> MACWPQLRLLLWKNLTFRRRQTCQLLLEVAWPLFIFLILISVRLSYPPYEQHECHFPNKAMPSAGTLPWVQGIICNANNPCFRYPTPGEAPGVVGNFNKSIVARLFSDARRLLLYSQKDTSMKDMRKVLRTLQQIKKSSSNLKLQDFLVDNETFSGFLYHNLSLPKSTVDKMLRADVILHKVFLQGYQLHLTSLCNGSKSEEMIQLGDQEVSELCGLPREKLAAAERVLRSNMDILKPILRTLNSTSPFPSKELAEATKTLLHSLGTLAQELFSMRSWSDMRQEVMFLTNVNS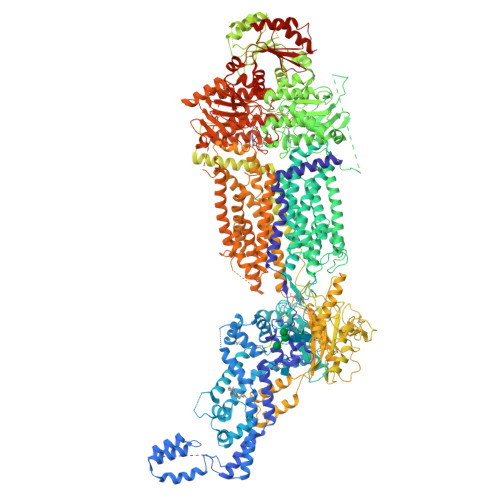SSSSTQIYQAVSRIVCGHPEGGGLKIKSLNWYEDNNYKALFGGNGTEEDAETFYDNSTTPYCNDLMKNLESSPLSRIIWKALKPLLVGKILYTPDTPATRQVMAEVNKTFQELAVFHDLEGMWEELSPKIWTFMENSQEMDLVRMLLDSRDNDHFWEQQLDGLDWTAQDIVAFLAKHPEDVQSSNGSVYTWREAFNETNQAIRTISRFMECVNLNKLEPIATEVWLINKSMELLDERKFWAGIVFTGITPGSIELPHHVKYKIRMDIDNVERTNKIKDGYWDPGPRADPFEDMRYVWGGFAYLQDVVEQAIIRVLTGTEKKTGVYMQQMPYPCYVDDIFLRVMSRSMPLFMTLAWIYSVAVIIKGIVYEKEARLKETMRIMGLDNSILWFSWFISSLIPLLVSAGLLVVILKLGNLLPYSDPSVVFVFLSVFAVVTILQCFLISTLFSRANLAAACGGIIYFTLYLPYVLCVAWRDYVGFTLKIFASLLSPVAFGFGCEYFALFEEQGIGVQWDNLFESPVEEDGFNLTTSVSMMLFDTFLYGVMTWYIEAVFPGQYGIPRPWYFPCTKSYWFGEESDEKSHPGSNQKRISEICMEEEPTHLKLGVSIQNLVKVYRDGMKVAVDGLALNFYEGQITSFLGHNGAGKTTTMSILTGLFPPTSGTAYILGKDIRSEMSTIRQNLGVCPQHNVLFDMLTVEEHIWFYARLKGLSEKHVKAEMEQMALDVGLPSSKLKSKTSQLSGGMQRKLSVALAFVGGSKVVILDQPTAGVDPYSRRGIWELLLKYRQGRTIILSTHHMDEADVLGDRIAIISHGKLCCVGSSLFLKNQLGTGYYLTLVKKDVESSLSSCRNSSSTVSYLKKEDSVSQSSSDAGLGSDHESDTLTIDVSAISNLIRKHVSEARLVEDIGHELTYVLPYEAAKEGAFVELFHEIDDRLSDLGISSYGISETTLEEIFLKVAEESGVDAETSDGTLPARRNRRAFGDKQSCLRPFTEDDAADPNDSDIDPESRETDLLSGMDGKGSYQVKGWKLTQQQFVALLWKRLLIARRSRKGFFAQIVLPAVFVCIALVFSLIVPPFGKYPSLELQPWMYNEQYTFVSNDAPEDTGTLELLNALTKDPGFGTRCMEGNPIPDTPCQAGEEEWTTAPVPQTIMDLFQNGNWTMQNPSPACQCSSDKIKKMLPVCPPGAGGLPPPQRKQNTADILQDLTGRNISDYLVKTYVQIIAKSLKNKIWVNEFRYGGFSLGVSNTQALPPSQEVNDAIKQMKKHLKLAKDSSADRFLNSLGRFMTGLDTKNNVKVWFNNKGWHAISSFLNVINNAILRANLQKGENPSHYGITAFNHPLNLTKQQLSEVALMTTSVDVLVSICVIFAMSFVPASFVVFLIQERVSKAKHLQFISGVKPVIYWLSNFVWDMCNYVVPATLVIIIFICFQQKSYVSSTNLPVLALLLLLYGWSITPLMYPASFVFKIPSTAYVVLTSVNLFIGINGSVATFVLELFTDNKLNNINDILKSVFLIFPHFCLGRGLIDMVKNQAMADALERFGENRFVSPLSWDLVGRNLFAMAVEGVVFFLITVLIQYRFFIRPRPVNAKLSPLNDEDEDVRRERQRILDGGGQNDILEIKELTKIYRRKRKPAVDRICVGIPPGECFGLLGVNGAGKSSTFKMLTGDTTVTRGDAFLNKNSILSNIHEVHQNMGYCPQFDAITELLTGREHVEFFALLRGVPEKEVGKVGEWAIRKLGLVKYGEKYAGNYSGGNKRKLSTAMALIGGPPVVFLDQPTTGMDPKARRFLWNCALSVVKEGRSVVLTSHSMEECEALCTRMAIMVNGRFRCLGSVQHLKNRFGDGYTIVVRIAGSNPDLKPVQDFFGLAFPGSVLKEKHRNMLQYQLPSSLSSLARIFSILSQSKKRLHIEDYSVSQTTLDQVFVNFAKDQSDDDHLKDLSLHKNQTVVDVAVLTSFLQDEKVKESYVGDYKDDDDK> GPPTTPKCIQCGQYLDDPDLKYGQHPPDAVDEPQMLTNEKLSIFDANESGFESYEALPQHKLTCFSVYCKHGHLCPIDTGLIEKNIELFFSGSAKPIYDDDPSLEGGVNGKNLGPINEWWITGFDGGEKALIGFSTSFAEYILMDPSPEYAPIFGLMQEKIYISKIVVEFLQSNSDSTYEDLINKIETTVPPSGLNLNRFTEDSLLRHAQFVVEQVESYDEAGDSDEQPIFLTPCMRDLIKLAGVTLGQRRAQARRQTIRHSTREKDRGPTKATTTKLVYQIFDTFFAEQIEKDDREDKENAFKRRRCGVCEVCQQPECGKCKACKDMVKFGGSGRSKQACQERRCPNMAMKEADDDEEVDDNIPEMPSPKKMHQGKKKKQNKNRISWVGEAVKTDGKKSYYKKVCIDAETLEVGDCVSVIPDDSSKPLYLARVTALWEDSSNGQMFHAHWFCAGTDTVLGATSDPLELFLVDECEDMQLSYIHSKVKVIYKAPSENWAMEGGMDPESLLEGDDGKTYFYQLWYDQDYARFESPPKTQPTEDNKFKFCVSCARLAEMRQKEIPRVLEQLEDLDSRVLYYSATKNGILYRVGDGVYLPPEAFTFNIKLSSPVKRPRKEPVDEDLYPEHYRKYSDYIKGSNLDAPEPYRIGRIKEIFCPKKSNGRPNETDIKIRVNKFYRPENTHKSTPASYHADINLLYWSDEEAVVDFKAVQGRCTVEYGEDLPECVQVYSMGGPNRFYFLEAYNAKSKSFEDPPNHARSPGNKGKGKGKGKGKPKSQACEPSEPEIEIKLPKLRTLDVFSGCGGLSEGFHQAGISDTLWAIEMWDPAAQAFRLNNPGSTVFTEDCNILLKLVMAGETTN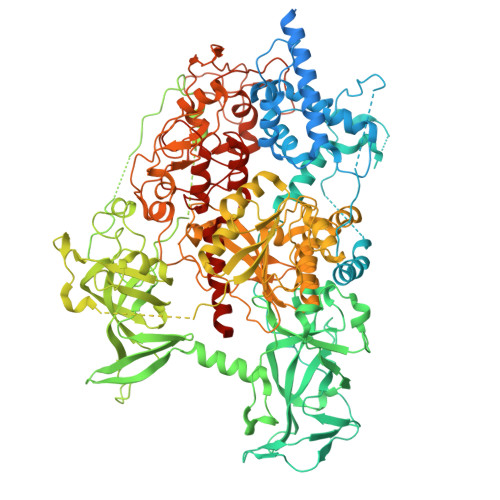SRGQRLPQKGDVEMLCGGPPCQGFSGMNRFNSRTYSKFKNSLVVSFLSYCDYYRPRFFLLENVRNFVSFKRSMVLKLTLRCLVRMGYQCTFGVLQAGQYGVAQTRRRAIILAAAPGEKLPLFPEPLHVFAPRACQLSVVVDDKKFVSNITRLSSGPFRTITVRDTMSDLPEVRNGASALEISYNGEPQSWFQRQLRGAQYQPILRDHICKDMSALVAARMRHIPLAPGSDWRDLPNIEVRLSDGTMARKLRYTHHDRKNGRSSSGALRGVCSCVEAGKACDPAARQFNTLIPWCLPHTGNRHNHWAGLYGRLEWDGFFSTTVTNPEPMGKQGRVLHPEQHRVVSVRECARSQGFPDTYRLFGNILDKHRQVGNAVPPPLAKAIGLEIKLCMLAKARESASAKIKEEEAAKD>MSLQGIHLSDLSYKHAILKESQYTIKRDVGTTTAVTPSSLQQEITLLCGEILYAKHADYKYAAEIGIQYISTALGSERVQQILRNSGSEVQVVLTRTYSLGKIKNNKGEDLQMLDIHGVEKSWVEEIDKEARKTMATLLKESSGNIPQNQRPSAPDTPIILLCVGALIFTKLASTIEVGLETTVRRANRVLSDALKRYPRMDIPKIARSFYDLFEQKVYHRSLFIEYGKALGSSSTGSKAESLFVNIFMQAYGAGQTMLRWGVIARSSNNIMLGHVSVQAELKQVTEVYDLVREMGPESGLLHLRQSPKAGLLSLANCPNFASVVLGNASGLGIIGMYRGRVPNTELFSAAESYAKSLKESNKINFSSLGLTDEEKEAAEHFLNVSDDSQNDYEKHHHHHH[12x]

The viral genome is encapsidated in a sheath of oligomerized copies of the nucleoprotein N, forming a ribonucleoprotein complex termed nucleocapsid. The nucleocapsid is the template for transcription and replication by L, which is also dependent on the obligate polymerase cofactor, the phosphoprotein P, together forming the active L/P holoenzyme. In oligomerized and RNA-bound N (N-RNA) the nucleic acid is threaded along an extended groove in between the NTDs and CTDs of laterally connected N protomers. An important function of the C-terminal domain of P in nsNSVs is to bind to assembled N-RNA, forming an N-RNA/P complex.

However, 11-mer oligomers (black arrow), 12-mer oligomers (white arrow), and short coil-like segments, denoted as spiral particles, are also present in the preparation (red arrow). Finally, 3D-reconstruction of the spiral particles yielded a coulomb potential map at an intermediate resolution of 4.7 Å. The map density of the spiral particle shows N protomers forming a spiral staircase and stacking up upon each other, in a mode reminiscent of a helical assembly. The map is most reliable in the central protomers and becomes increasingly disordered towards the outer protomers. As the map quality was globally too limited for atomic refinement we restricted ourselves to rigid-body placement of N-RNA protomers. We were able to rigid body fit 12 protomers of N into the map. Thresholding of the map at a low level indicates the presence of additional N protomers, however, this density was too diffuse to fit more copies of N, presumably due to heterogeneity of the sample or conformational heterogeneity. It is notable that in this arrangement the RNA strand is obscured by N protomers belonging to the next turn of the assembly, suggesting that a conformational change is necessary for the genome to become accessible to L/P. Taking together our cryo-EM reconstructions, we observe that the lateral interaction of RNA-bound N protomers can support a range of geometries, demonstrating the plasticity of N-RNA and supporting the notion of a highly flexible HMPV nucleocapsid.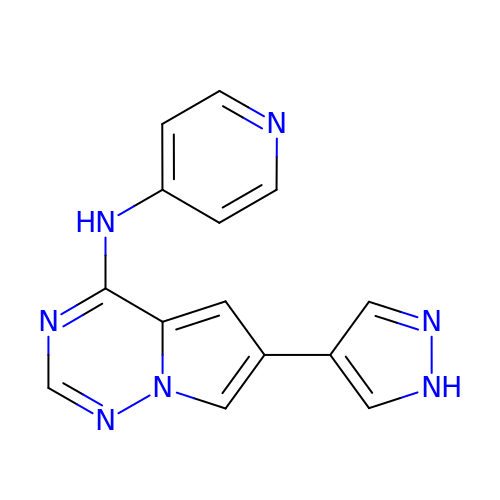6-(1H-pyrazol-4-yl)-N-(pyridin-4-yl)pyrrolo[2,1-f][1,2,4]triazin-4-amine | C14 H11 N7 | KFPMWFGUHKKDSW-UHFFFAOYSA-N>MSKLLMIGTGPVAIQLANICYLKSDYEIDMVGRASTSEKSKRLYQAYKKEKQFEVKIQNEAHQHLEGKFEINRLYKDVKNVKGEYETVVMACTADAYYDTLQQLSLETLQSVKHVILISPTFGSQMIVEQFMSKFSQDIEVISFSTYLGDTRIVDKEAPNHVLTTGVKKKLYMGSTHSNSTMCQRISALAEQLKIQLEVVESPLHAETRNSSLYVHPPLFMNDFSLKAIFEGTDVPVYVYKLFPEGPITMTLIREMRLMWKEMMAILQAFRVPSVNLLQFMVKENYPVRPETLDEGDIEHFEILPDILQEYLLYVRYTAILIDPFSQPDENGHYFDFSAVPFKQVYKNEQDVVQI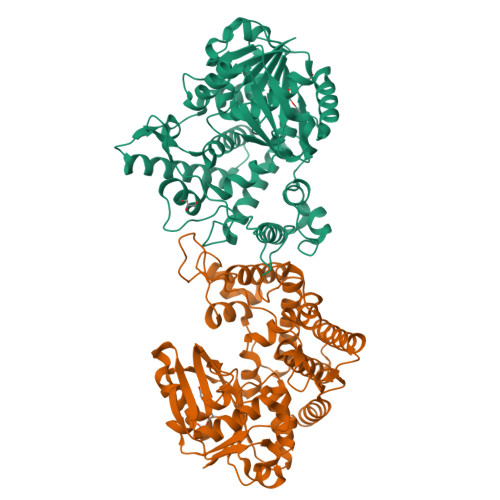PRMPSEDYYRTAMIQHIGKMLGIKTPMIDQFLTRYEASCQAYKDMHQDQQLSSQFNTNLFEGDKALVTKFLEINRTLSLEHHHHHH[2x]>MKKLALIALPLVLASCTMAGPTEGTYTLAPQAVVKPAGPVYAPAGTAKISETLGVTRTTITLTGMAPYAIYVAHYHKMGTAAPMGSAPATNTNMAMSSTDATATTTASTSTTSTDTTVAASTDMTTTVTMAPVTAAPNPCNSDGPAIMESRMIAQASADGKVTLTGIVPTALIRDAAYINVHHGRDFSGALADSGVICTPITMTMR[3x]

The S-layer Deinoxanthin-binding complex (SDBC), one of the main units of the characteristic multilayered cell envelope of this bacterium, protects against environmental stressors and allows exchanges with the environment. The crystalline cell envelope/S-layer of D. radiodurans is made by three different multisubunit protein complexes among which the main one is the S-layer Deinoxanthin-binding complex (SDBC), composed of the xanthophyll-binding protein DR_2577 (SlpA) and at least five more accessory subunits. The SDBC appeared to be composed of three main regions: (i) a massive β-barrel organization structuring the pores' region, (ii) a β-sandwich organization characterizing the collar region, and (iii) a trimeric coiled coil for the stalk region. The SDBC is shown to be both a photoprotective system, through the xanthophyll-binding subunit DR_2577, and a chemoprotective one, by the SOD activity of the subunit DR_0644.

The collar region of the SDBC was solved by cryo-EM at ∼2.5 Å resolution and found to consist of a single protein complex organized as a trimer. The protein sequence was modeled assigning 120 residues, missing a central threonine-rich region between the residues 90 and 137, which could be either disordered or truncated with respect to its ORF. Two short and disordered parts of the sequence, flanking the cleaved region upstream (residues 80–89) and downstream (residues 138–141), as well as a small N-terminal region interacting with the xanthophyll carotenoid deinoxanthin, remained unassigned (Leu6-Ala19). The DR_0644 presents a typical β-sandwich motif, with six opposing antiparallel β-sheets, creating a structure with a width of ∼34 Å and a length of ∼85 Å. The three monomers assemble into a trimer via a linking region of 17 residues at the N-terminal side (Gly20 – Pro36). Bioinformatic analysis by basic local alignment indicated the DR_0644 to be a SOD while metal ion-binding site prediction and docking studies (MIB) allowed us to localize a single Cu-binding site for each SOD monomer. The Cu-binding site involves three characteristic His residues (His74, His76, and His182), indicating DR_0644 to be a Cu-only SOD, a group of soluble enzymes typical for the periplasm and extracellular compartments and here unusually found to be part of a cell envelope complex, the SDBC. Coordination and distances for the assigned binding site supported the presence of Cu2+. The lower resolution of the collar allowed to identify and assign the Cu-binding domain but not to localize the densities for the Cu ions, which were predicted with high confidence by different bioinformatic means. The characteristic active site with the three coordinated histidines structurally confirmed the Cu-only SOD identity of this protein, corroborating the function of the collar region.> MGSSHHHHHHQWNVSLQPPPQQLIVQNKTIDLPAVYQLNGGEEANPHAVKVLKELLSGKQSSKKGMLISIGEKGDKSVRKYSRQIPDHKEGYYLSVNEKEIVLAGNDERGTYYALQTFAQLLKDGKLPEVEIKDYPSVRYRGVVEGFYGTPWSHQARLSQLKFYGKNKMNTYIYGPKDDPYHSAPNWRLPYPDKEAAQLQELVAVANENEVDFVWAIHPGQDIKWNKEDRDLLLAKFEKMYQLGVRSFAVFFDDISGEGTNPQKQAELLNYIDEKFAQVKPDINQLVMCPTEYNKSWSNPNGNYLTTLGDKLNPSIQIMWTGDRVISDITRDGISWINERIKRPAYIWWNFPVSDYVRDHLLLGPVYGNDTTIAKEMSGFVTNPMEHAESSKIAIYSVASYAWNPAKYDTWQTWKDAIRTILPSAAEELE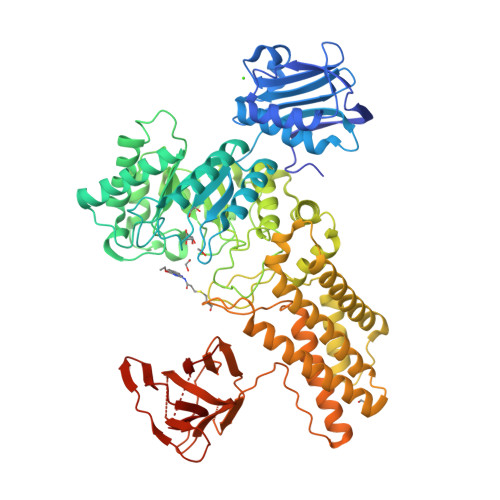SFAMHNSDLGPNGHGYRREESMDIQPAAERFLKAFKEGKNYDKADFETLQYTFERMKESADILLMNTENKPLIVEITPWVHQFKLTAEMGEEVLKMVEGRNESYFLRKYNHVKALQQQMFYIDQTSNQNPCQPGVKTATRVIKPLIDRTFATVVKFFNQKFNAHLDATTDYMPHKMISNVEQIKNLPLQVKANRVLISPANEVVKWAAGNSVEIELDAIYPGENIQINFGKDAPSTWGRLEISTDGKEWKTVDLKQKESRLSAGLQKAPVKFVRFTNVSDEEQQVYLRQFVLTIEKK> QYVRIKNWGSGEILHDTLHHKATS;> SCLGSIMNPKSLTRGPRDKPTPLEELLPHAIEFINQYYGSFKEAKIEEHLARLEAVTKEIETTGTYQLTLDELIFATKMAWRNAPRCIGRIQWSNLQVFDARNCSTAQEMFQHICRHILYATNNGNIRSAITVFPQRSDGKHDFRLWNSQLIRYAGYQMPDGTIRGDAATLEFTQLCIDLGWKPRYGRFDVLPLVLQADGQDPEVFEIPPDLVLEVTMEHPKYEWFQELGLKWYALPAVANMLLEVGGLEFPACPFNGWYMGTEIGVRDFCDTQRYNILEEVGRRMGLETHTLASLWKDRAVT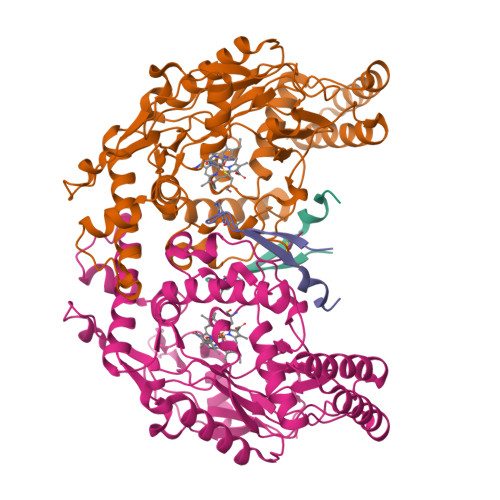EINVAVLHSFQKQNVTIMDHHTASESFMKHMQNEYRARGGCPADWIWLVPPVSGSITPVFHQEMLNYVLSPFYYYQIEPWKTHIWQ>[6x]MTTGGPLAGVKVIELGGIGPGPHAGMVLADLGADVVRVRRPG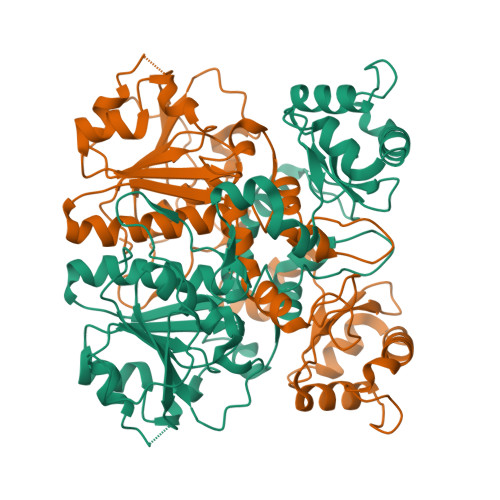GLTMPSEDRDLLHRGKRIVDLDVKTQPQAMLELAAKADVLLDCFRPGTCERLGIGPDDCASVNPRLIFARITGWGQDGPLASTAGHDINYLSQTGALAAFGYADRPPMPPLNLVADFGGGSMLVLLGIVVALYERERSGVGQVVDAAMVDGVSVLAQMMWTMKGIGSLRDQRESFLLDGGAPFYRCYETSDGKYMAVGAIEPQFFAALLSGLGLSAADVPTQLDVAGYPQMYDIFAERFASRTRDEWTRVFAGTDACVTPVLAWSEAANNDHLKARSTVITAHGVQQAAPAPRFSRTPAGPVRPPPAAATPIDEINW Nylon hydrolase (NylC) is one of the three enzymes responsible for the endo-type degradation of the by-products of nylon-6 manufacture (cyclic and linear oligomers of 6-aminohexanoate (Ahx) with a degree of polymerization greater than three) and various aliphatic nylons (e.g., nylon-6 and nylon-66). However, the post-translational autocleavage of the nascent polypeptide between Asn266 and Thr267 generates an active enzyme with an α subunit (27 kDa) and a β subunit (9 kDa). Based on the X-ray-crystallographic structure of NylCA, we reported that four αβ heterodimers (molecules A-D) form a doughnut-shaped quaternary structure. In addition, we proposed that the nucleophilic N-terminal residue Thr267 in the β subunit functions as a catalytic residue for either autocleavage (from precursor to active enzyme) or substrate hydrolysis.

In contrast, the MAV of wild-type NylCp2 was 85,602 based on sedimentation equilibrium analysis. For example, in wild-type NylCp2 (Asp122, Tm = 52.9 °C), the distance between position 112 (monomer A) and position 122 (monomer D) at Cα (designated as “a1”) was 7.04 Å. In contrast, the distance between position 122 (monomer A) and position 112 (monomer D) (designated as “a2”) was considerably greater with a value of 8.43 Å. In contrast, NylCp2 existed at the monomer/dimer/trimer equilibrium in aqueous solution (2.1 S, 2.7 S, and 3.5 S). Thus, it was likely that the partial asymmetry at the A/D interface disrupted tetramer formation (reaction 2) but generated an irregular trimeric structure in aqueous solution by reaction 3 or by successive reactions (reaction 2 followed by reaction 8), although the enzyme was identified to be a tetramer by the crystallographic analysis described above. In wild-type NylCp2, Lys159-NH3+ (located on helix α2 in molecule A) was 2.87 Å away from Glu115-Oε1− (located on helix α1 in molecule D). However, in NylCp2, the amino acid residue at position 122 was replaced with Asp, and the close proximity of the acidic residue Asp122 (close to Glu115) reduced this stabilization effect. However, the structures of loop 1 and loop 3 containing His130 in NylCp2 were not built during X-ray-crystallographic analysis due to the poor electron density. Moreover, the temperature factors (index of thermal motion in a crystallographic structure) of loop regions 1–3 in NylCp2 were significantly larger than those of the corresponding regions in the thermostable NylC-G122Y130 mutant.

>MNTTPVHALTDIDGGIAVDPAPRLAGPPVFGGPGNDAFDLAPVRSTGREMLRFDFPGVSIGAAHYEEGPTGATVIHIPAGARTAVDARGGAVGLSGGYDFNHAICLAGGAGYGLEAGAGVSDALLERLEHRTGFAELQLVSSAVIYDFSARSTAVYPDKALGRAALEFAVPGEFPQGRAGAGMSASAGKVDWDRTEITGQGAAFRRLGDVRILAVVVPNPVGVIVDRAGTVVRGNYDAQTGVRRHPVFDYQEAFAEQVPPVTEAGNTTISAIVTNVRMSPVELNQFAKQVHSSMHRGIQPFHTDMDGDTLFAVTTDEIDLPTTPGSSRGRLSVNATALGAIASEVMWDAVLEAGK[2x]> MGSSNTVTSAVKTQYVEIESVDGFYFNTEDKFDTAQIKKAVLHTVYNEGYTGDDGVAVVLREYESEPVDITAELTFGDATPANTYKAVENKFDYEIPVYYNNATLKDAEGNDATV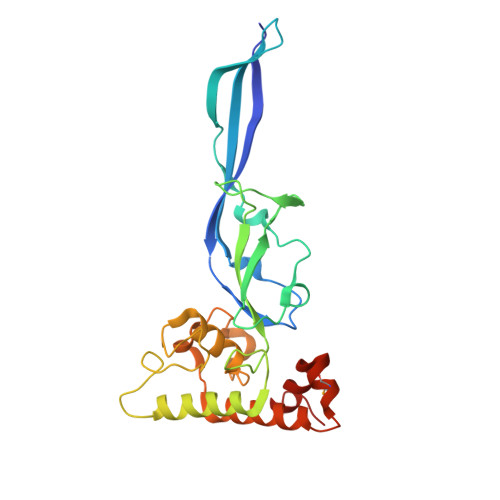TVYIGLKGDTDLNNIVDGRDATATLTYYAATSTDGKDATTVALSPSTLVGGNPESVYDDFSAFLSDVKVDAGKELTRFAKKAERLIDGRDASSILTFYTKSSVDQYKDMAANEPNKLWDIVTGDAEEE>GPGSVSRVSREELEDRFLRLHDENILLKQHARKQED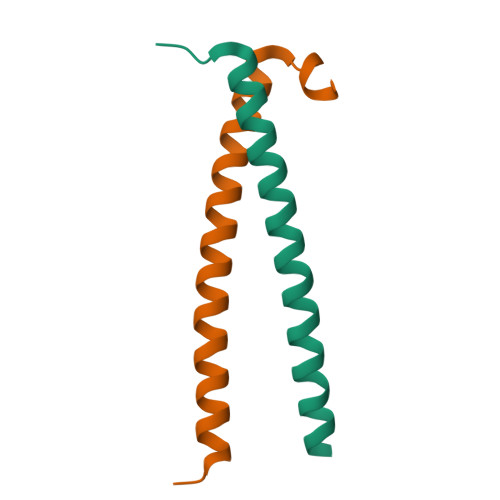KIKRMATKLIRLVNDKKRYERVGG[4x]> MVKRKSSEGQEQDGGRGIPLPIQTFLWRQTSAFLRPKLGKQYEASCVSFERVLVENKLHGLSPALSEAIQSISRWELVQAALPHVLHCTATLLSNRNKLGHQDKLGVAETKLLHTLHWMLLEAPQDCNNDQFGGTDRGSSWGGSSSAFIHQIENQGSPGQPCRSSSHDEEENNRRKTFQNSMATVELFVFLFAPLVHRIKESDLTFRLASGLVIWQPMWEHRQPEVSGFTALVKPIRNIITAKRSSPINSQSQTCESPNQDTRQQGEGLQVVSEALQSDSISPKATISGCHQGNSFDGSLSSQTSQERGPSHSRASLVIPPCQRSRYATYFDVAVLRCLLQPHWSEEGTQWSLMYYLQRLRHMLEEKPEKTPDPDIPLLPRPRSSSMVAAAPSLVNTHKTQDLTMKCNEEEKSLSPEAFSKVSLTNLRRSAVPDLSSDLGMNIFKKFKSRKEDRERKGSIPFHHTGKRRPRRMGVPFLLHEDHLDVSPTRSTFSFGSFSGLGEDRRGIEKGGWQTTILGKLTRRGSSDAATEMESLSARHSHSHHTLVSDLPDHSNSHGENTVKEVRSQISTITVATFNTTLASFNVGYADFFSEHMRKLCSQVPIPEMPHEPLACANLPRSLTDSCINYSYLEDTEHIDGTNNFVHKNGMLDLSVVLKAVYLVLNHDISSRICDVALNIVECLLQLGVVPCVEKNRKKSENKENESVEKRPSEGAFQFKGVSSSSTSGFGAPSASGAGDGGGEEGGGGDGGGGGGGGDGGGGGGGGGGPYEKNEKNQEKDDNIPVSNHRLALTMLIKIVKSLGCAYGCGEGHRGLSGDRLRHQVFRENAQNCLTKLYKLDKIQFRQTMRDYVNKDSLNNVVDFLHALLGFCMEPVTDNKAGFGNNFTTVDNKSTAQNVEGIIVGAMFKSLITRCASTTHELHSPENLGLYCDIRQLVQFIKEAHGNVFRRVALSALLDSAEKLAPGKKVEENGQESKPVGSKRSEAGSIADKGQVSSAPEECRSFMSGRPSQTPEHDEPMQGGNLGRKDFWRKMFKSQSAASDTSSQSEQDTSECTTAHSGNTSDRRARSRSRRISLRKKLKLPIGNWLKRSSLSGLADGVEDLLDISSVDRLSFIRQSSKVKFTSAVKLSEGGPGSGMENGREEEENFFKRLGCHSFDDHLSPNQDGGKSKNVVNLGAIRQGMKRFQFLLN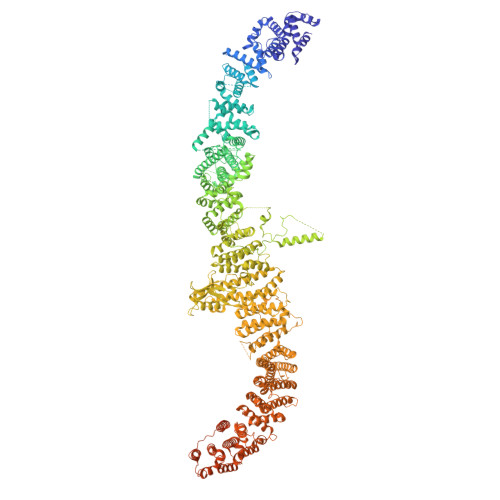CCEPGTIPDASILAAALDLEAPVVARAALFLECARFVHRCNRGNWPEWMKGHHVNITKKGLSRGRSPTVGNKRNQKLQWSAAKLFYQWGDAIGIRLNELCHGESESPANLLGLIYDEETKRRLRKEDEEEDFLDDSTVNPSKCGCPFALKMAACQLLLEITTFLRETFSCLPRPRTEPLVDLESCRLRLDPELDRHRYERKISFAGVLDENEDSKDSLHSSSHTIKSDAGAEEKKVPSRKIRIGGSRLLQIKGTRSFQVKKGGSLSSIRRVGSLKSSKLSRQDSESEAEELQLSQSRDTVTDLEGSPWSASEPSIEPEGLSNAGTEENYHRNMSWLHVMILLCNQQSFICTHVDYCHPHCYLHHSRSCARLVRAIKLLYGDSVDSLRESNHISNVALRGKKQKECSDKSCLRTPSLKKRVSDVNLEGKKDSGMLKYIRFQVMSLSPAPLSLLIKAAPILTEEMYGDIQPAAWELLLSMDEHMAGAAAAMFLLCAVKVPDAVSDMLMSEFHHAETVQRLNAVLKFHTLWRFRYQVWPRMEEGAQQIFKIPPPSINFTLPSPVLGMPSVPMFDPPWVPQCSGSVQDPINEDQSKSFSARAVSRSHQRAEHILKNLQQEEEKKRLGREASLITAIPITQEACYEPTCTPNSEPEEEEEVANLTSRRLSVSPSCTSSTSHRNYSFRRGSVWSVRSAVSAEDEEHATEHTPNHHVPQPPQAVFPACICAAVLPIVHLMEDGEVREDGVAVSAVAQQVLWNCLIEDPSTVLRHFLEKLTISNRQDELMYMLRKLLLNIGDFPAQTSHILFNYLVGLIMYFVRTPCEWGMDAISATLTFLWEVVGYVEGLFFKDLKQTMKKEQCEVKLLVTASMPGTKTLVVHGQNECDIPTQLPVHEDTQFEALLKECLEFFNIPESQSTHYFLMDKRWNLIHYNKTYVRDIYPFRRSVSPQLNLVHMHPEKGQELIQKQVFTRKLEEVGRVLFLISLTQKIPTAHKQSHVSMLQEDLLRLPSFPRSAIDAEFSLFSDPQAGKELFGLDTLQKSLWIQLLEEMFLGMPSEFPWGDEIMLFLNVFNGALILHPEDSALLRQYAATVINTAVHFNHLFSLSGYQWILPTMLQVYSDYESNPQLRRAIEFACHQFYILHRKPFVLQLFASVAPLLEFPDAANTGSSKGVSAQCLFDLLQSLEGETTDILDILELVKAEKPLKSLDFCYGNEDLTFSISEAIKLCVTVVAYAPESFRSLQMLMVLEALVPCYLQKMKRQTSQVETVPAAREEIAATAALATSLQALLYSVEVLTRPMTAPQMSRSDQGHKGTTTANHTMSSGVNTRYPEQGAKLHFIRENLHLLEEGQGLPREELDERISREEFRRPRESLLNICTEFYKHCGPRLKILQNLAGEPRVTALELLDVKSHMRLAEIAHSLLKLAPYDTQTMESRGLRRYIMEMLPITDWSAEAVRPALILILKRLDRMFNKIHKMPTLRRQVEWEPASSLIEGVCLTLQRQPIISFLPHLRSLINVCVNLVMGVVGPSSVADGLPLLHLSPYLSPPLPFSTAVVRLVALQIQALKEDFPLSHVISPFTNQERREGMLLNLLIPFVLTVGSGSKDSPWLEQPEVQLLLQTVINVLLPPRIISTSRSKNFMLESSPAHCSTPGDAGKDLRKEGLAESTSQAAYLALKVILVCFERQLGSQWYWLSLQVKEMALRKVGGLALWDFLDFIVRTRIPIFVLLRPFIQCKLLAQPAENHEELSARQHISDQLERRFIPRPLCKSSLIAEFNSELKILKEAVHSGSAYQGKTSISTVGTSTSAYRLSLATMSRSNTGTGTVWEQDSEPSQQASQDTLSRTDEEDEENDSVSMPSVVSEQEACLLSTIGRRRFSSHVSSMSAPQAEVGMLPSQSEPNVLDDSQGLAAEGSLSRVASIQSEPGQQNVLLQQPLGRKRGLRQLRRPLLSRQKTQTEPRNRHGARLSTTRRSIQPKTKPSVDQKRSVTFIEAQPEPTAAPTDIFPATGQPQSCSPGRARKPEGTEKPVLTSSPAIIIADLHSLSPKQSEPLLAEEGEKKEDEEIQGATAHCPLSTQLSDPDDFTGLETSSLLQHGDTVLHISEENGTENPLLSSQFTFTPPELGDTDSALDESHV> GSHMSGIALSRLAQERRAWRKDHPFGFVAVPTKNPDGTMNLMNWECAIPGKKGTPWEGGLFKLRMLFKDDYPSSPPKCKFEPPLFHPNV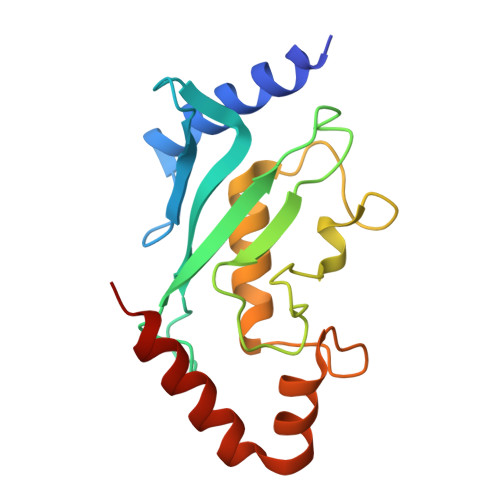YPSGTVCLSILEEDKDWRPAITIKQILLGIQELLNEPNIQDPAQAEAYTIYCQNRVEYEKRVRAQAKKFAPS PML belongs to the TRIM family of proteins, defined by the presence of a RING domain, one or two other zinc fingers and a long coiled coil. PML RING, B boxes and coiled coil are all important for NB-biogenesis. PML NBs also recruit enzymes implicated in several post-translational modifications, primarily UBC9, the key E2 SUMO-conjugating enzyme, possibly facilitating partner sumoylation. Here we report the crystallographic high-resolution structure of PML RING, and demonstrate that it assembles into a tetrameric torus.

We have determined the crystal structure of PML RING at a 1.6 Å resolution by single wavelength anomalous dispersion. Similar to previous RING structures, the folding of PML RING49–104 is coordinated by two Zn ions, but in contrast with previous studies, PML RING leads tetrameric complexes. Within a tetramer, each PML subunit adopts a balloon shape configuration with two distinct sub-domains. Sub-domain 1 (SD1FQF) is a loop containing only three residues, F52Q53F54, while sub-domain 2 (SD2), comprising residues 55–99, is a classic C3HC4 RING finger. Together with homo-dimerization of SD2, interactions between SD1FQF and SD2 create a four subunits torus-like structure. Within the current tetramer, the N-terminal F52Q53F54 SD1FQF undergoes a radical 23 Å swing away from the adjacent SD2, allowing the SD1FQF loop to engage with the hydrophobic pocket of the other subunit. This shift also exposes L73 and allows SD2 dimerization. As estimated by the AREAIMOL25 program, the buried surfaces between one set of SD1FQF/SD2 and SD2/SD2 dimers are 1333 and 779 Å2, respectively. As oligomerization proceeds, the buried surface of PML RING tetramer increases significantly to 4216 Å2, accounting for ~40% of the overall surface of PML RING tetramer.

>EEEFQFLRCQQCQAEAKCPKLLPCLHTLCSGCLEASGMQCPICQAPWPLGA[4x]>[6x]MGSDKIHHHHHHVIIESRIEKGKPVVGMETTVFVHGLPRKEAIE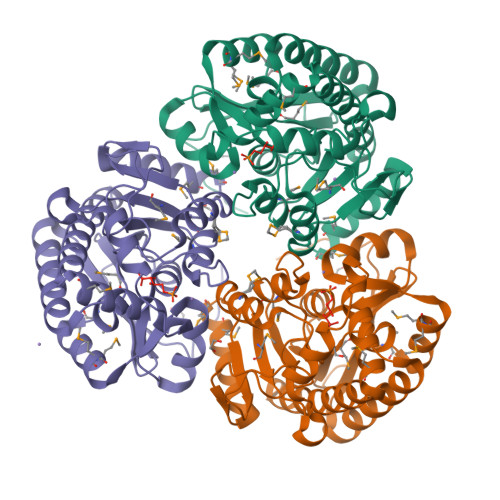LFRRAKEISREKGFQLAVIGILKGKIVAGMSEEELEAMMREGADKVGTREIPIVVAEGKNAATTVSATIFLSRRIGIEVVVTGGTGGVHPGRVDVSQDLTEMSSSRAVLVSSGIKSILDVEATFEMLETLEIPLVGFRTNEFPLFFSRKSGRRVPRIENVEEVLKIYESMKEMELEKTLMVLNPVPEEYEIPHDEIERLLEKIELEVEGKEVTPFLLKKLVEMTNGRTLKANLALLEENVKLAGEIAVKLKRS> MTGAVCPGSFDPVTLGHVDIFERAAAQFDEVVVAILVNPAKTGMFDLDERIAMVKESTTHLPNLRVQVGHGLVVDFVRSCGMTAIVKGLRTGTDFEYELQMAQMNKHIAGVDTFFVATAPRYSFVSSSLAK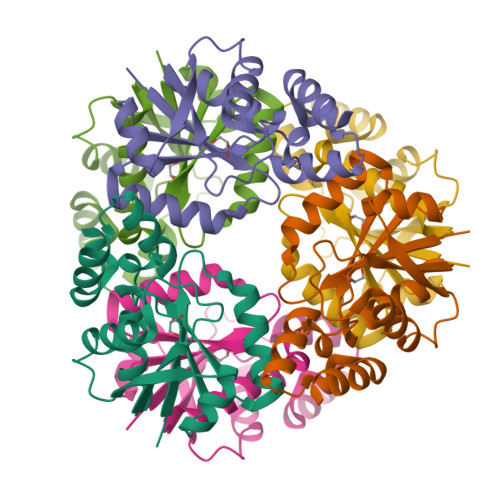EVAMLGGDVSELLPEPVNRRLRDRLNTERT> MIYVTFTPYGAFGVKDNKEVSGLEDIEYKKLFNEEEIPDIMFKLKTQPNKIADELKEEWGDEIKLETLSTEPFNI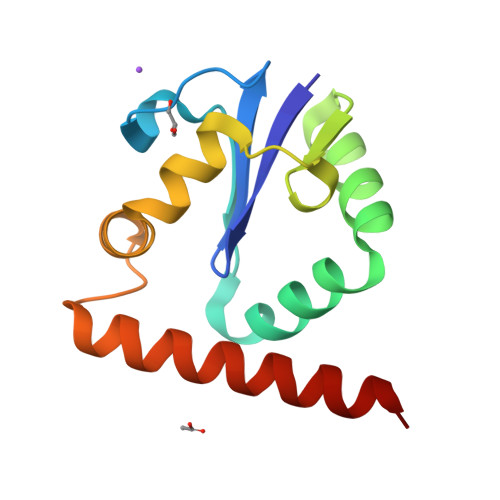GEFLRNNLFKVGKELGYFNNYDEFRKKMHYWSTELTKKVIKSYA> SSVVVDTNGQPVSNGADAYYLVPVSHGHAGLALAKIGNEAEPRAVVLDPHHRPGLPVRFESPLRINIIKESYFLNIKFGPSSSDSGVWDVIQQDPIGLAVKVTDTKSLLGPFKVEK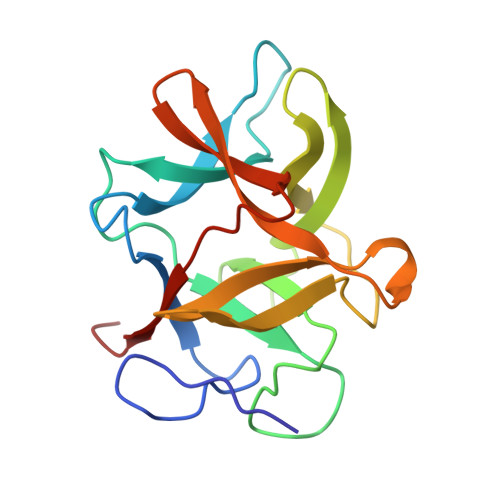EGEGYKIVYYPERGQTGLDIGLVHRNDKYYLAVKDGEPCVFKIRKATDE Death-associated protein kinase (DAPK) is a member of the Ca2+/calmodulin-regulated family of serine/threonine protein kinases. The role of the kinase activity of DAPK in eukaryotic cell apoptosis and the ability of bioavailable DAPK inhibitors to rescue neuronal death after brain injury have made it a drug-discovery target for neurodegenerative disorders. The three DAPK conformations demonstrate that nucleotide binding brings about changes in conformation that are mostly localized to the glycine-rich loop region. The most notable conformational changes occur in the glycine-rich loop region, an active-site region with potential for modulation of kinase activity.

Therefore, we determined a new crystal structure of DAPK–AMP-PNP–Mg2+ using a combination of cocrystallization of DAPK with AMP-PNP and MgCl2 followed by soaking of crystals in a cryoprotection solution that contained AMP-PNP and MgCl2, similar to the method used to obtain the DAPK–ADP–Mg2+ complex. The DAPK–AMP-PNP–Mg2+ crystals grew in a high concentration of ammonium sulfate and diffracted to 2.00 Å resolution. c OMIT map contained clear density for the nucleotide, including the β- and γ-phosphates and one magnesium ion. The positioning of the γ-phosphate in the new DAPK–AMP-PNP–Mg2+ structure is such that it is in a ‘kinked’ conformation similar to that observed in other kinase–AMP-PNP structures such as PKA, JNK3, GSK3β, CDK2 and phosphorylase kinase. Initial modeling and refinement revealed partial negative density located around the γ-phosphate of the nucleotide, despite the use of the highest purity nucleotide available (see §2). The adjustment of the occupancies of the γ-­phosphate and the OG1, O2G and O3G atoms to 0.60 resulted in elimination of the negative density in the refinement model, thereby allowing a comparative analysis between nucleotide-bound states. The improved density of the γ-phosphate of AMP-PNP allows a closer examination of protein atoms that are within hydrogen-bonding distance of the γ-­phosphate atoms and also those atoms within proximity that might be involved in the phospho-transfer process. The only protein atom that is within potential hydrogen-bonding distance is Asp139 OD1 (2.8 Å). In the AMP-PNP structure, the Mg2+ ion makes fewer interactions with the protein residues and only coordinates to Asp161 OD2, while other inter­actions are made with the O1A atom of the α-­phosphate, the O3G and O2G atoms of the γ-phosphate and a water molecule. The r.m.s. deviation for these residues between apo DAPK and DAPK–AMP-PNP–Mg2+ is 1.03 Å and that between apo DAPK and DAPK–ADP–Mg2+ is 0.62 Å.

> MTVFRQENVDDYYDTGEELGSGQFAVVKKCREKSTGLQYAAKFIKKRRTKSSRRGVSREDIEREVSILKEIQHPNVITLHEVYENKTDVILILELVAGGELFDFLAEKESLTEEEATEFLKQILNGVYYLHSLQIAHFDLKPENIMLLDRNVPKPRIKIIDFGLAHKIDFGNEFKNIFGTPEFVAPEIVNYEPLGLEADMWSIGVITYILLSGASPFLGDTKQETLANVSAVNYEFEDEYFSNTSALAKDFIRRLLVKDPKKRMTIQDSLQHPWIKPKDTQQALSSAWSHPQFEK>[4x]LVDLSFE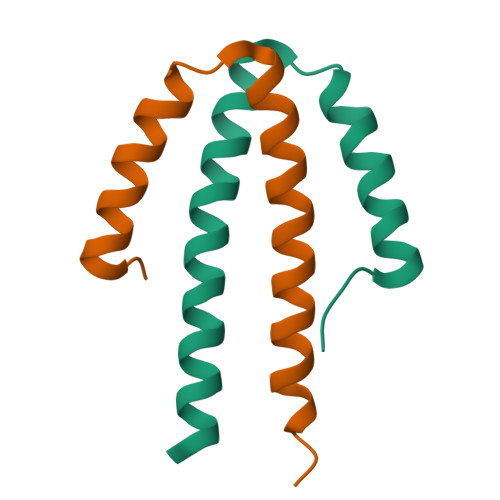QEFQMRVMEEQVSAMSLQEARELLLQASRLLMMKDNVIRSLVKRAAR> MVMNKQIVLNNYINGSLKQSDLALRTSTICMEIPDGCNGAILVKNLYLSVNPYLILRMGKLDIPQFDSILPGSTIVSYGVSKVLDSTHPSYEKGELIWGSQAGWEEYTLIQNPYNLFKIQDKDVPLSYYVGILGMPGMTAYAGFFEICSPKKGETVFVTAAAGSVGQLVGQFAKMFGCYVVGSAGSKEKVDLLKNKFGFDDAFNYKEESDYDTALKRHFPEGIDIYFDNVGGKMLEAVINNMRVHGRIAVCGMVSQYSLKQPEGVHNLLKLIPKQIRMQGFVVVDYYHLYPKFLEMVLPRIKEGKVTYVEDISEGLESAPSALLGVYVGRNVGNQVVAVSRE

Pulegone reductase is the key enzyme in the biosynthesis of menthol and is required for the stereoselective reduction of the Δ2,8 double bond of pulegone to produce the major intermediate menthone, thus determining the stereochemistry of menthol. Pulegone reductase is a double bond reductase (DBR) which belongs to the NADPH-dependent, medium-chain dehydrogenase/reductase (MDR) superfamily. In Mentha piperita, (−)-menthone is directly synthesized from (+)-pulegone through the reduction of C2–C8 alkene double bond catalyzed by (+)-pulegone reductase (EC number 1.3.1.81). Some DBRs in the MDR superfamily proteins have become important biotechnological tools for asymmetric synthesis due to their high stereoselectivity in the alkene double bond reduction. It has been reported that the reduction reaction proceeds through stereoselective transfer of a hydride from NADPH to the carbon of the substrate.

In this study, we characterized a novel (−)-pulegone reductase from Nepeta tenuifolia (NtPR), which can catalyze (−)-pulegone to (+)-menthone and (−)-isomenthone through our RNA-seq, bioinformatic analysis in combination with in vitro enzyme activity assay, and determined the structure of (+)-pulegone reductase from M. piperita (MpPR) by using X-ray crystallography, molecular modeling and docking, site-directed mutagenesis, molecular dynamics simulations, and biochemical analysis. Phylogenetic analysis revealed both NtPR and MpPR belong to the MDR superfamily, but they are present in two different clades. To investigate the structural basis and underlying mechanism of the stereoselectivity, we performed molecular docking, molecular dynamic simulation, site-directed mutagenesis analysis, and biochemical assays based on the crystal structure of MpPR. We identified and validated the critical residues in the crystal structure of MpPR involved in the binding of the substrate pulegone. We also further identified that residues Leu56, Val282, and Val284 determine the stereoselectivity of the substrate pulegone, and mainly contributes to the product stereoselectivity. We uncovered the key residues in the pulegone binding pockets of NtPR and MpPR, and illustrated that the hydrophobic interactions and potential steric hindrances may mainly contribute to their stereoselectivity toward substrates and products. This study not only deepens our understanding on the substrate and product selectivity of alkene reductases, but also provides a structural and mechanistic basis for the engineering and directed evolution of pulegone reductases, enabling the production of enantiomerically pure end-product in industry.> MAKWVCKICGYIYDEDAGDPDNGISPGTKFEELPDDWVC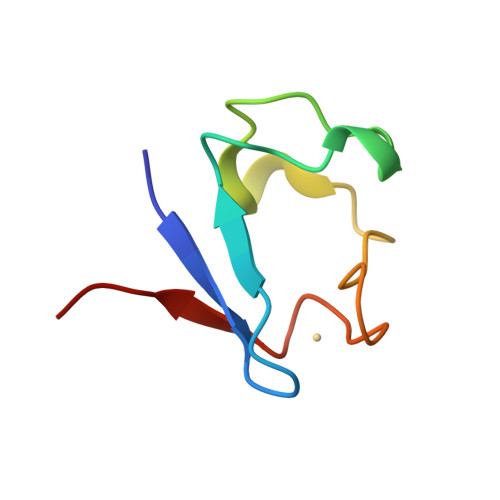PICGAPKSEFEKLED> SNAIAVGSERSADGKGMLLANPHFPWNGAMRFYQMHLTIPGRLDVMGASLPGLPVVNIGFSRHLAWTHTVDTSSHFTLYRLALDPKDPRRYLVDGRSLPLEEKSVAIEVRGADGKLSRVEHKVYQSIYGPLVVWPGKLDWNRSEAYALRDANLENTRVLQQWYSINQASDVADLRRRVEALQGIPW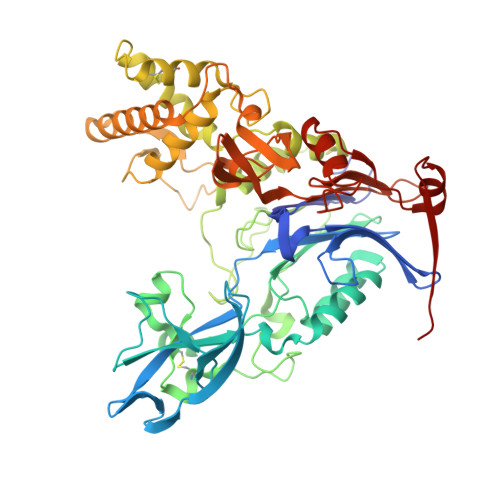VNTLAADEQGNALYMNQSVVPYLKPELIPACAIPQLVAEGLPALQGQDSRCAWSRDPAAAQAGITPAAQLPVLLRRDFVQNSNDSAWLTNPASPLQGFSPLVSQEKPIGPRARYALSRLQGKQPLEAKTLEEMVTANHVFSADQVLPDLLRLCRDNQGEKSLARACAALAQWDRGANLDSGSGFVYFQRFMQRFAELDGAWKEPFDAQRPLDTPQGIALDRPQVATQVRQALADAAAEVEKSGIPDGARWGDLQVSTRGQERIAIPGGDGHFGVYNAIQSVRKGDHLEVVGGTSYIQLVTFPEEGPKARGLLAFSQSSDPRSPHYRDQTELFSRQQWQTLPFSDRQIDADPQLQRLSIREAA9-cis-okenone | C41 H54 O2 | 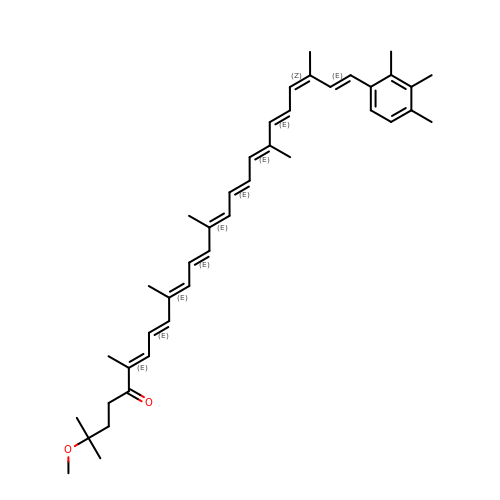FSQZIFSGNDUYRQ-KKGQYTAFSA-N>[2x]MSGSRPTQSSEGSRRSRHSARIIAQTTVDAKLHADFEESGSSFDYSTSVRVTGPVVENQPPRSDKVTTTYLHHIQKGKLIQPFGCLLALDEKTFKVIAYSENASELLTMASHAVPSVGEHPVLGIGTDIRSLFTAPSASALQKALGFGDVSLLNPILVHCRTSAKPFYAIIHRVTGSIIIDFEPVKPYEVPMTAAGALQSYKLAAKAITRLQSLPSGSMERLCDTMVQEVFELTGYDRVMAYKFHEDDHGEVVSEVTKPGLEPYLGLHYPATDIPQAARFLFMKNKVRMIVDCNAKHARVLQDEKLSFDLTLCGSTLRAPHSCHLQYMANMDSIASLVMAVVVNEEDGEGDAPDATTQPQKRKRLWGLVVCHNTTPRFVPFPLRYACEFLAQVFAIHVNKEVELDNQMVEKNILRTQTLLCDMLMRDAPLGIVSQSPNIMDLVKCDGAALLYKDKIWKLGTTPSEFHLQEIASWLCEYHMDSTGLSTDSLHDAGFPRALSLGDSVCGMAAVRISSKDMIFWFRSHTAGEVRWGGAKHDPDDRDDARRMHPRSSFKAFLEVVKTRSLPWKDYEMDAIHSLQLILRNAFKDSETTDVNTKVIYSKLNDLKIDGIQELEAVTSEMVRLIETATVPILAVDSDGLVNGWNTKIAELTGLSVDEAIGKHFLTLVEDSSVEI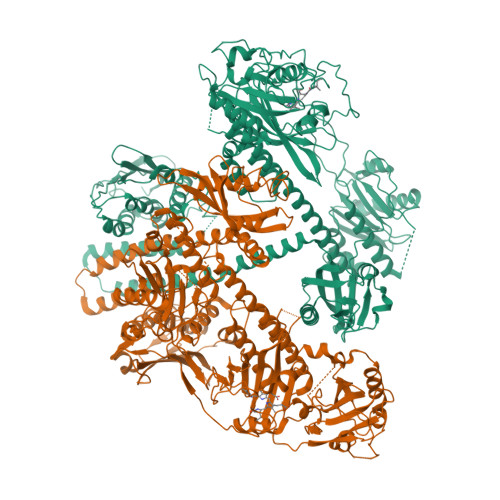VKRMLENALEGTEEQNVQFEIKTHLSRADAGPISLVVNACASRDLHENVVGVCFVAHDLTGQKTVMDKFTRIEGDYKAIIQNPNPLIPPIFGTDEFGWCTEWNPAMSKLTGLKREEVIDKMLLGEVFGTQKSCCRLKNQEAFVNLGIVLNNAVTSQDPEKVSFAFFTRGGKYVECLLCVSKKLDREGVVTGVFCFLQLASHELQQALHVQRLAERTAVKRLKALAYIKRQIRNPLSGIMFTRKMIEGTELGPEQRRILQTSALCQKQLSKILDDSDLESIIEGCLDLEMKEFTLNEVLTASTSQVMMKSNGKSVRITNETGEEVMSDTLYGDSIRLQQVLADFMLMAVNFTPSGGQLTVSASLRKDQLGRSVHLANLEIRLTHTGAGIPEFLLNQMFGTEEDVSEEGLSLMVSRKLVKLMNGDVQYLRQAGKSSFIITAELAAANK One specific mechanism used by nairoviruses is the production of a deubiquitinating enzyme, termed the vOTU, that disrupts the innate immune response. Interestingly, the nairoviral L segment also encodes a viral homologue of the ovarian tumor protease (OTU) at the N-terminus. Instead, the vOTU’s primary function appears to be the reversal of post-translational modifications by ubiquitin (Ub) and the Ub-like protein interferon stimulated gene product 15 (ISG15). Each vOTU possesses a seven-stranded beta sheet as the core feature, with five major alpha helices framing the rest of the structure.

Similar to the pattern observed for HAZV and GANV, QYBV vOTU shows the most activity towards K11, though at lower overall levels. Additionally, QYBV vOTU shows a more pronounced difference in the relative preference for K48 versus K63 linkages, with substantially more activity towards K48. In QYBV vOTU, Trp72 packs with Pro85. Additionally, it is in proximity to His79, suggesting potential stacking of the rings. Specifically, direct interactions, or the lack thereof, work in conjunction with the other interactions to complete the structural features. This is most notable in QYBV vOTU, in which Phe14 appears to pack with Pro76. In contrast, the DGKV and QYBV vOTUs possess more polar residues, including asparagine, glutamate, and threonine for DGKV and glutamine and lysine in QYBV. Despite being phylogenetically distant from CCHFV and the other robust vOTU DUBs, QYBV demonstrates substantial Ub activity and possesses Ile130 that could pack with Ub’s Leu8. Further, increasing the hydrophobicity of the pocket in QYBV vOTU was able to enhance Ub-AMC cleavage, boosting activity by 150% and 50% for the Q19V and Q128A mutants, respectively.

>MANLKENIVWEHVFDNCSQANVVFSYREFFNKELTLPDGNCFFRAVSTFLYDTQNGWIEVKNMCREFAETNWDELPGVHQYFQDPEHYARESKREGYWGGSVEAEILSKLLKLTVIFWKCEDDVWVTQGIRWGDGNYLTAINLLHIQFDHFDFLVPINVTQEPPKSGSHHHHHH[3x]>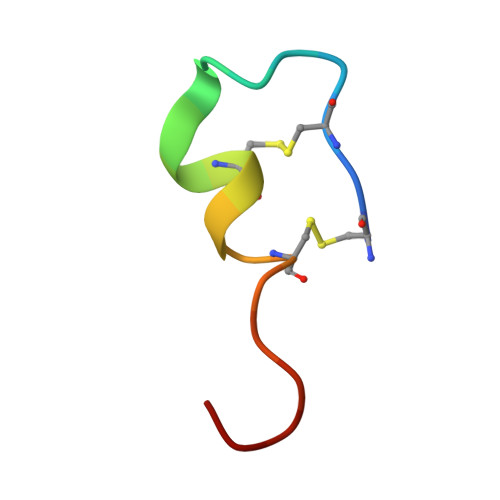[2x]CSCSSLMDKECVYFCHLDIIW The housecleaning enzyme of Mycobacterium tuberculosis (Mtb), MazG, is a nucleoside triphosphate pyrophosphohydrolase (NTP-PPase) and can hydrolyze all canonical or non-canonical NTPs into NMPs and pyrophosphate. The Mycobacterium tuberculosis MazG (Mtb-MazG) contributes to antibiotic resistance in response to oxidative or nitrosative stress under dormancy, making it a promising target for treating TB in latent infection patients. As a housecleaning enzyme, MazG functions at the cell nucleotide metabolism by degrading the non-canonical NTPs, preventing mutagenesis and DNA damage. Mtb-MazG mainly contains three domains, an extra N-terminal region (NE, residues 1–85) that is absent in other bacterial homologs, the N-terminal domain (NTD, residues 86–253), and the C-terminal domain (CTD, residues 254–325; Mota et al., 2016).

Despite failing in the crystallization of full-length MazG, we succeeded in obtaining the MazG (1–185) protein crystals and solved the 2.7 Å resolution structure using molecular replacement of the AlphaFold2-predicted structure (AF-P96379-F1). There are six MazG molecules in an asymmetrical unit with a cell dimension of 109 × 109 × 242 Å, which includes two monomers and two dimers consisting of two identical chains. The Mtb-MazG (1–185) monomer contained eight α-helices and five β-stands, comprising two globular domains, including a primary three-layered α/β/α sandwich domain (named domain 1) and an entirely α-helices-composed domain (named domain 2). Domain 1 was composed of three α-helices (α1, α2, and α3) and five β-sheet strands (β1, β2, β3, β4, and β5), which was absent in other NTP pyrophosphatases, including B. anthracis, E. coli, and D. radiodurans MazGs. Domain 2 included five α-helices (α4, α5, α6, α7, and α8), which showed a higher B-factor than that in domain 1, indicating this region exhibited more flexibility. The two domains were connected with a short linker (Ala78-Gly84). The interface-involved residues of the swapped-dimeric MazG were located in α1 of domain 1, and α4, α6, and α8 of domain 2, of which fifteen residues formed multiple hydrogen bonds and salt bridges in relative distances within 3.5 Å. In the MazG (1–185) structure, one magnesium ion was present per subunit. The Mg2+ was coordinated by three glutamate residues (Glu119, Glu122, and Glu138) and one aspartate (Asp141). Also, the NTP-PPase activity was significantly lowered for the mutants of E119A, E122A, E138A, and D141A.

>[6x]MIVVLVDPRRPTLVPVEAIEFLRGEVQYTEEMPVAVPWSLPAARSAHAGNDAPVLLSSDPNHPAVITRLAAGARLISAPDSQRGERLVDAVAMMDKLRTAGPWESEQTHDSLRRYLLEETYELLDAVRSGSVDQLREELGDLLLQVLFHARIAEDASQSPFTIDDVADTLMRKLGNRAPGVLAGE>MKCIVGLGNIGKRFELTRHNIGFEVVDYILEKNNFSLDKQKFKGAYTIERMNGDKVLFIEPMTMMNLSGEAVAPIMDYYNVNPEDLIVLYDDLDLEQGQVRLRQKGSAGGHNGMKSIIKMLGTDQFKRIRIGVGRPTNGMTVPDYVLQRFSNDEMVTMEKVIEHAARAIEKFVE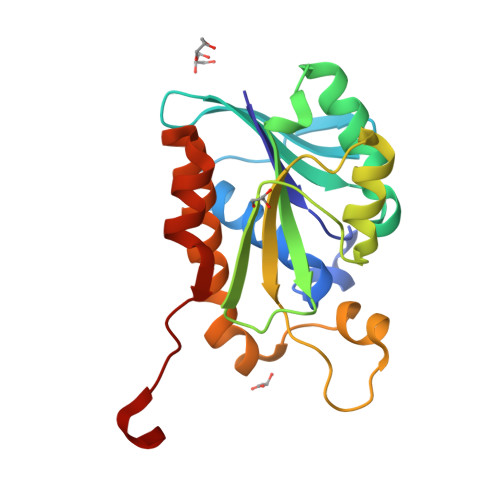TSRFDHVMNEFNGEVKLEHHHHHH[2x]> IEMKPHPWFFGKIPRAKAEEMLSKQRHDGAFLIRESES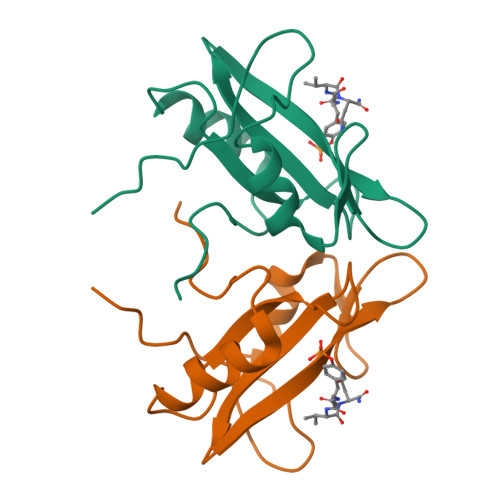APGDFSLSVKFGNDVQHFKVLRDGAGKYFLWVVKFNSLNELVDYHRSTSVSRNQQIFLRDIEQVPQQPTYVQHHHHHH> MQQQCDTVSAWQSLRGPGTGGYYLFKTTEGGKTDCTYVKGSNFNDAAQTATYTYGNLGSGNQLTQQTASASISGNAIVVGTDHSEVLYSDGSTCDVVRLNGQIELWIHSSATSNTGNLNSCCTDKFNQEKG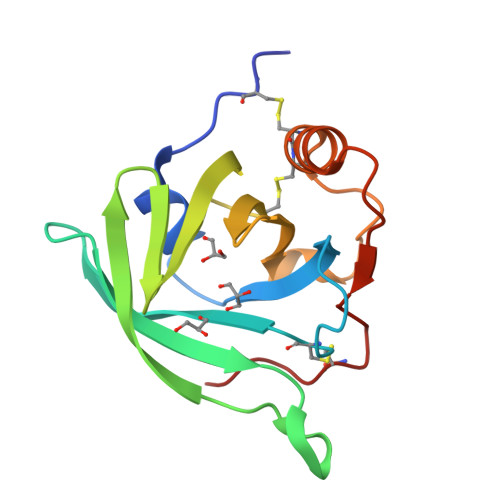SRPEHVVYRSTCPNLPA> NQIVSGAAWTDTAGNTIQ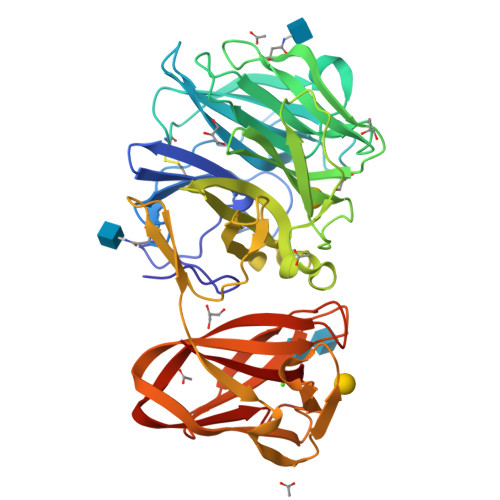AHGAGILQVGSTFYWFGEDKSHNSALFKAVSCYTSSDLVNWSRQNDALSPIAGTMISTSNVVERPKVIFNQKNSEYVMWFHSDSSNYGAAMVGVATAKTPCGPYTYKGSFKPLGADSRDESIFQDDDSAQTAYLLYASDNNQNFKISRLDANYYNVTAQVSVMNGATLEAPGIVKHNGEYFLIASHTSGWAPNPNKWFSASSLAGPWSAQQDIAPSATRTWYSQNAFDLPLGSNAIYMGDRWRPSLLGSSRYIWYPLDFSSGAPQIVHADVWSVNVQAGTYSVASGTSYEAENGQRGGSSTILSGSGFSGGKAVGYLGHGGTVTINNVQSNGGSHWVALYFANGDSTYRNVTVSVNGGPSVLVDQPDSGGGNVVISVPVKLNLNSGENSITFGSGQSNYAADLDKIIVY> SPSAEACGYS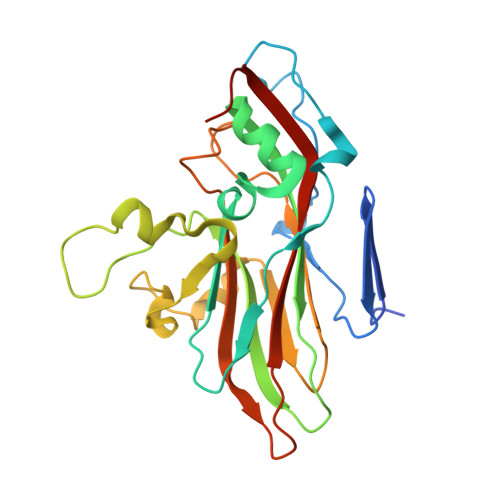DRVLQLKLGNSAIVTQEAANYCCAYGEWPNYLPDHEAVAIDKPTQPETSTDRFYTLRSVKWESNSTGWWWKLPDALNNIGMFGQNVQYHYLYRSGFLIHVQCNATKFHQGALLVVAIPEHQRGAHDTTTSPGFNDIMKGERGGTFNHPYVLDDGTSIACATIFPHQWINLRTNNSATIVLPWMNVAPMDFPLRHNQWTLAVIPVVPLGTRTMSSVVPITVSIAPMCCEFNGLRHAITQ> 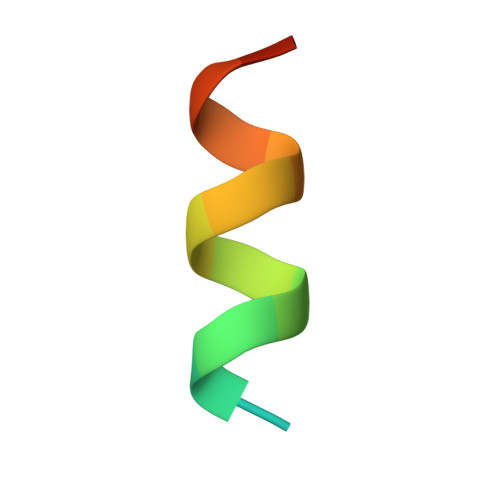DDKLQKWVRVYLDRGQ> ATCDDGRTTANAACCILFPILDDIQENLFDGAQCGEEVHESLRLTFHDAIGFSPTLGGGGADGSIIAFDTIETNFPANAGIDEIVSAQKPFVAKHNISAGDFIQFAGAVGVSNCP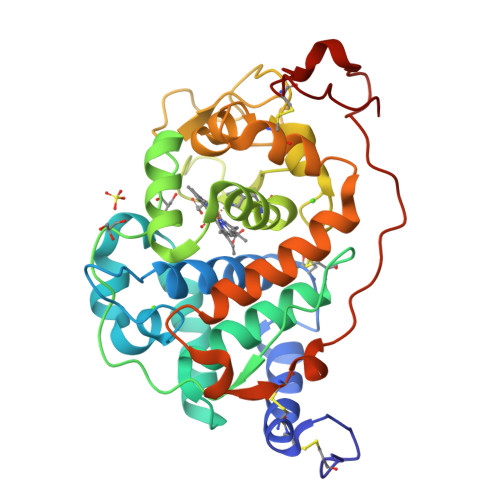GGVRIPFFLGRPDAVAASPDHLVPGPFDSVDSILARMGDAGFSPVEVVWLLASHSIAAADKVDPSIPGTPFDSTPEVFDSQFFIETQLKGRLFPGTADNKGEAQSPLQGEIRLQSDHLLARDPQTACEWQSMVNNQPKIQNRFAATMSKMALLGQDKTKLIDCSDVIPTPPALVGAAHLPAGFSLSDVEQACAATPFPAL(5S,7R,8S,9S,10R)-8,9,10-trihydroxy-7-(hydroxymethyl)-2-thioxo-6-oxa-1,3-diazaspiro[4.5]decan-4-one 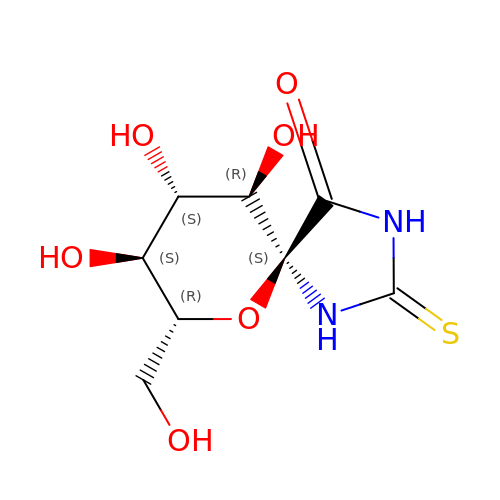| C8 H12 N2 O6 S | OEWLGQKSTDZKFN-WWHASAIZSA-N>MGSSHHHHHHSSGRENLYFQGHMDIKACYQNAKALLEGHFLLSSGFHSNYYLQSAKVLEDPKLAEQLALELAKQIQEAHLNIECVCSPAIGGILAGYELARALGVRFIFTERVDNTMALRRGFEVKKNEKILVCEDIITTGKSAMECAKVLEEKGAQIVAFGALANRGICKRAHSH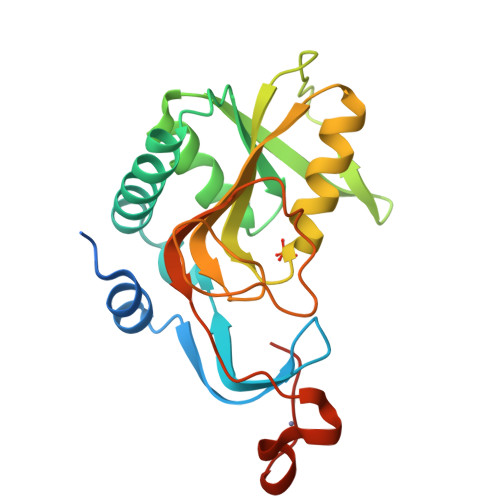LKAQEGACLPSHLPLFALEDFVFDMHKPSSCPLCATSVAIKPGSRGNGS[2x]> MEKSFVITDPRLPDNPIIFASDGFLELTEYSREEILGRNGRFLQGPETDQATVQKIRDAIRDQREITVQLINYTKSGKKFWNLLHLQPMRDQKGELQYFIGV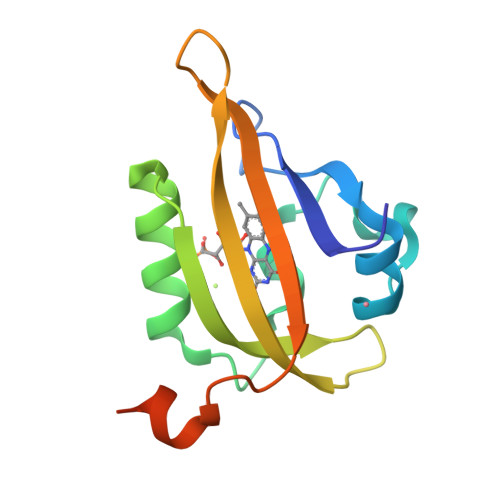LLDGEFIPNPLLGLDSTRTGHHHHHH> GVQVPDVRGQSSADAIATLQNRGFKIRTLQKPDSTIPPDHVIGTDPAANTSVSAGDEITVNVSTGPEQREIPDVSTLTYAEAVKKLTAA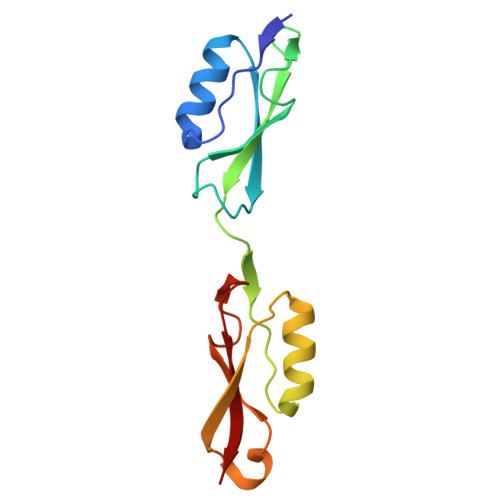GFGRFKQANSPSTPELVGKVIGTNPPANQTSAITNVVIIIVGSG80α is a typical example of a staphylococcal transducing phage, capable of transferring non-specific chromosomal or plasmid DNA at low frequency. The capsids are assembled from a major capsid protein (CP) as empty precursor procapsids into which the DNA is packaged through the portal by the phage terminase. Many SaPIs, such as SaPI1, redirect the 80α capsid assembly pathway to form capsids that are smaller than the normal phage capsids and that are thus incapable of packaging full-length phage genomes. Here, we report the structures of a mature 80α capsid made from an uncleavable version of CP at 5.2 Å resolution and of a wildtype SaPI1 mature capsid at 8.4 Å resolution.

The structure of the DNA-filled SaPI1 mature capsid was determined to 8.4 Å resolution using AUTO3DEM from 6471 particles picked from these images. The SaPI1 mature capsid displayed the expected T = 4 icosahedral architecture comprised of A5 pentamers and (BCD)2 hexamers located on fivefold and twofold symmetry axes, respectively. CP subunits A–D derived from the 80α CPFA model were placed into the SaPI1 density by rigid body fitting, followed by real-space refinement in Coot. Density for the N-arm was apparent, demonstrating that the extended conformation seen in the CPFA capsid was not due to the lack of CP cleavage. The distribution of CP subunits within hexamers, however, is dramatically different in the 80α and SaPI1 capsids. In the SaPI1 capsid, CP subunits on opposite sides of the hexamer are >11 Å further apart than in 80α, leaving a larger hole in the middle of the hexamer, and the hexamer has a distinct bend of ≈10° relative to 80α. These differences presumably reflect the different environments of the hexamers in the T = 7 and T = 4 capsids. In the T = 7 80α capsids, the hexamers are located on the flat face of the icosahedron, whereas in the T = 4 SaPI1 capsids, they sit on the twofold axis at the edges between faces. In the T = 4 SaPI1 shell, there is no rippling of hexamers around the threefold axis, and the dihedral angles α and β are identical to those observed in the procapsid. In this case, the distinctly different environment of the hexamer on the twofold axis is accommodated by changes in the hexamer itself.

>[4x]MEQTQKLKLNLQHFASNNVKPQVFNPDNVMMHEKKDGTLMNEFTTPILQEVMENSKIMQLGKYEPMEGTEKKFTFWADKPGAYWVGEGQKIETSKATWVNATMRAFKLGVILPVTKEFLNYTYSQFFEEMKPMIAEAFYKKFDEAGILNQGNNPFGKSIAQSIEKTNKVIKGDFTQDNIIDLEALLEDDELEANAFISKTQNRSLLRKIVDPETKERIYDRNSDSLDGLPVVNLKSSNLKRGELITGDFDKLIYGIPQLIEYKIDETAQLSTVKNEDGTPVNLFEQDMVALRATMHVALHIADDKAFAKLVPADKRTDSVPGEV>SLINTKIKPFKNQAFKNGEFIEVTEKDTEGRWSVFFFYPADFTFVCPTQLGDVADHYEELQKLGVDVYSVSTDTHFTHKAWHSSSETIAKIKYAMIGDPTGALTRNFDNMREDEGLADRATFVVDPQGIIQAIEVTAEGIGRDASDLLRKIKAAQYVAAHPGEVCPAKWKEGEA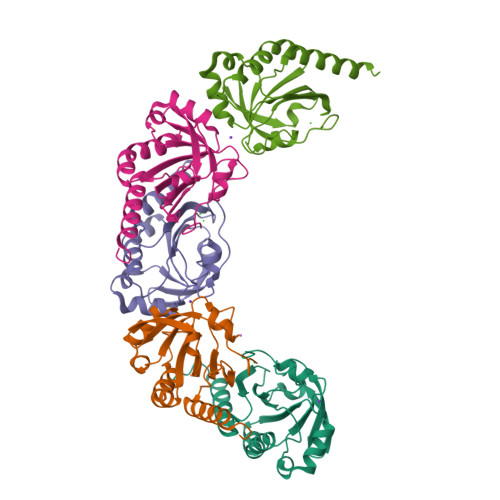TLAPSLDLVGKI[5x]> GTLSNRASK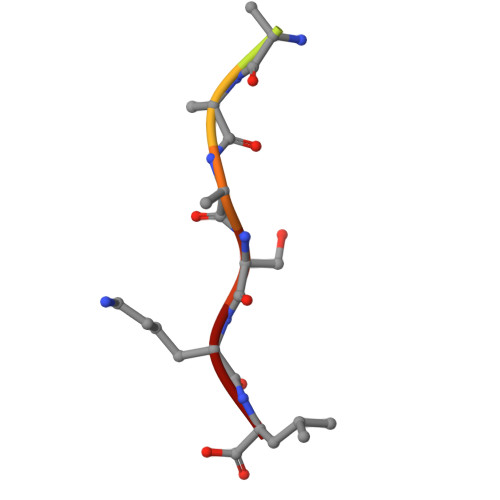L> DPSKDSKAQVSAAEAGITGTWYNQLGSTFIVTAGADGAL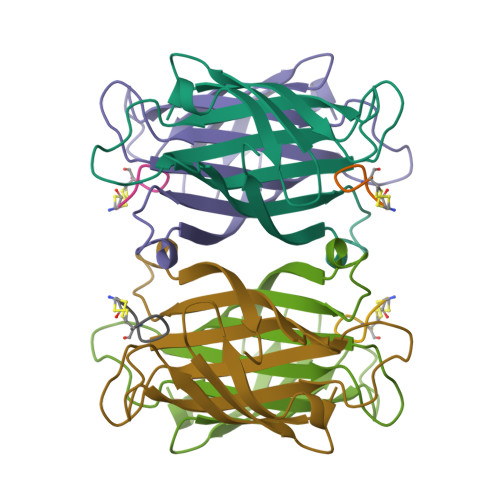TGTYESAVGNAESRYVLTGRYDSAPATDGSGTALGWTVAWKNNYRNAHSATTWSGQYVGGAEARINTQWLLTSGTTEANAWKSTLVGHDTFTKVKP> VTDYSGSGVKDFVFEVHRGDTTKVIGQRLKDEGVVATPSAFTDAAAGNQAIAAIQPGFYKLRTKIAGKEAVARLAEQDNRVGLLVIPEGRQLDDVSAVSNGAVTEGIFTLIARASCVDLDGDKHCVAASDLRQAATTASQGELDVPDWASNGVNAVRDDHRRIEGLIAAGRWDFDPMAEPEQILASLIRESNAQYQQLGLLSSDAAGLSPYQVLVVASLLQREAKPRDFAKVARVVYNRLAKHQKLEFDSTVNYPLDRQEVATTDEDRERKTLWNTYVSQGLSGTPISSPSPEALQAAERPEPGDWLYFVTIDAEGTTLFTADYNEHLANIELAKKNGILDSAR

One type of enzyme involved in this process is membrane-bound glycosidase, which cleaves the PG sugar backbone. Lytic transglycosyl­ase (LT), anchored to the cytoplasmic membrane, is a representative glycosidase enzyme that catalyzes nonhydrolytic cleavage of the β-1,4 glycosidic bond between MurNAc and GlcNAc to produce muropeptide products containing a 1,6-anhydro-MurNAc (anhMurNAc) end [Fig. 1(a)]. In a previous study, MltG was characterized as the terminase responsible for achieving PG integration into the cell wall through cleavage of the newly synthesized glycan strand. MltG consists of three domains: an N-terminal TMD, a predicted PG-binding domain and a C-terminal YceG (MltG) catalytic domain.

To obtain a soluble protein for studying the structure of maMltG, we constructed an N-terminal truncated version of the MltG expression vector, in which the N-terminal 84 residues of MltG (i.e. the TMD) were removed. The purified maMltG protein was crystallized and the 2.2 Å high-resolution crystal structure of maMltG was solved using the MR phasing method. A single maMltG molecule was identified in the asymmetric crystallographic unit. Thus, we believe that maMltG exists as a monomer in solution based on the SEC and MALS results. However, there is a huge structural discrepancy in the various locations of the PG-binding domain, indicating structural plasticity between the two domains of the MltG family.> AKPIEVTDQNFDETLGQHPLVLVDFWAEWCAPCRMIAPILEEIAKEYEGKLLVAKLDVDENPKTAMRYRVMSIPTV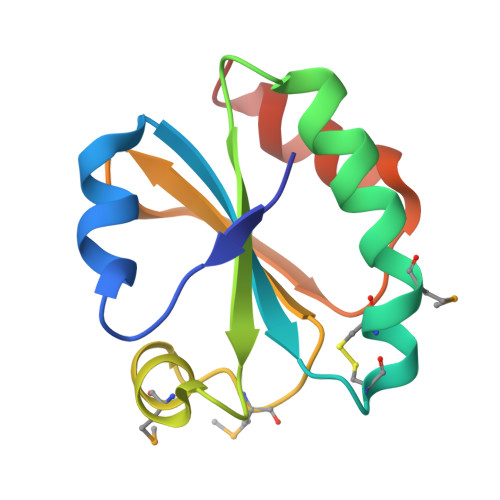ILFKDGQPVEVLVGAQPKRNYQAKIEKHLPATA>MQDEVVLLDFWPSPFGMRVRIALAEKGIKYEYKEEDLQNKSPLLLKMNPVHKKIPVLIHNGKPICESLIAVQYIEEVWNDRNPLLPSDPYQRAQTRFWADYVDKKIYDLGRKICTSKGEEKEAAKKEFIEALKLLEEQLGDKTYFGGDNLGFVDIALVPFYTWFKAYETFGTLNIESECPKFV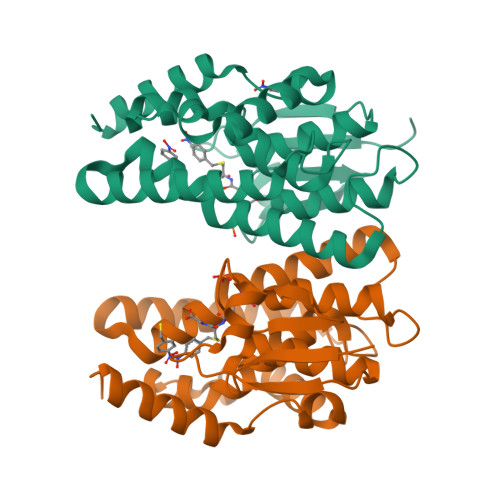AWAKRCLQKESVAKSLPDQQKVYEFIMDLRKKLGIE[2x]>DKATIPSESPFAAAEVADGAIVVDIAKMKYETPELHVKVGDTVTWINREAMPHNVHFVAGVLGEAAL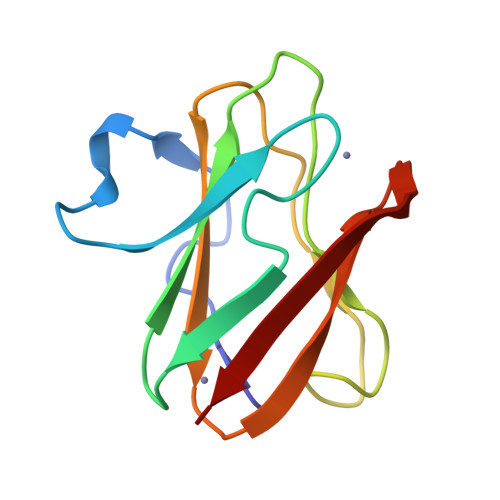KGPMMKKEQAYSLTFTEAGTYDYHCTPHPFKRGKVVVE[4x]>[2x]ASREQTMENILKAAKKKFGERGYEGTSIQEIAKEAKVNVAMASYYFNGKENLYYEVFKKYGLANELPNFLEKNQFNPINALREYLTVFTTHIKENPEIGTLAYE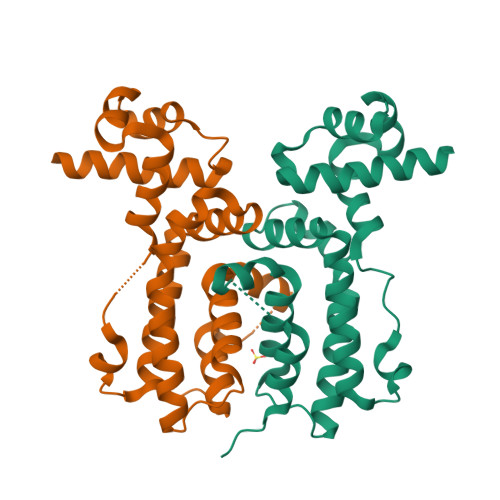EIIKESARLEKIKPYFIGSFEQLKEILQEGEKQGVFHFFSINHTIHWITSIVLFPKFKKFIDGSSGSSGLVSRIISALTDKPNI(2S,4aR,6R,7R,7aS)-6-[6-amino-8-(benzylsulfanyl)-9H-purin-9-yl]-2-sulfanyltetrahydro-4H-furo[3,2-d][1,3,2]dioxaphosphinin-7-ol 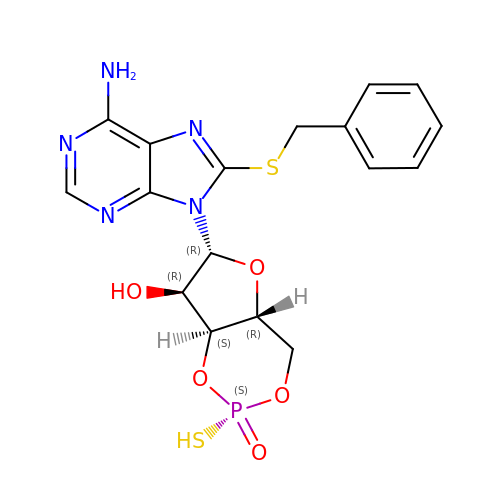2-oxide | C17 H18 N5 O5 P S2 | CXSXQZZDDPUUEA-LXJUGQNYSA-N> YSQPS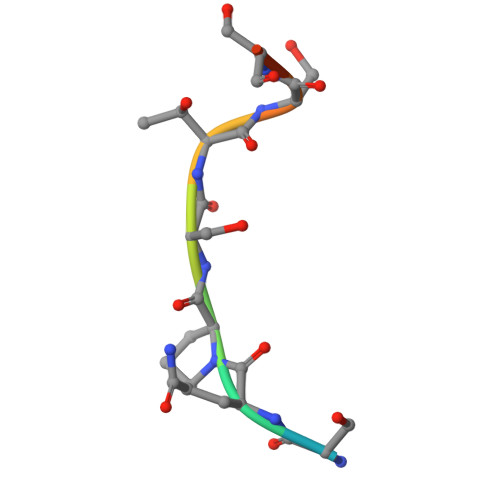TSSSI Gyrase is a type II topoisomerase and the only enzyme that can catalyse the introduction of negative supercoils into DNA;3,5 it is composed of two subunits, GyrA and GyrB, which form an A2B2 complex in the active enzyme. Gyrase is an essential enzyme in bacteria and has been extensively studied as a target for antibacterial agents;6 gyrase has been described as an effective drug target for the development of new anti-TB agents. Other compounds, such as the aminocoumarins (e.g. novobiocin), inhibit gyrase through targeting the ATPase domains of gyrase and topo IV, located in the N-terminal domain of GyrB (and ParE), thus preventing supercoiling. In addition, we present crystal structures of the GyrB N-terminal ATPase sub-domain from Mycobacterium thermoresistibile bound to one of these compounds (Redx03863) and also to novobiocin, demonstrating that this novel compound class inhibits via a binding pocket and resistance mechanism different from that of novobiocin.

Using cross-seeding from crystals of the novobiocin complex, crystals of Redx03863 bound to the 21 kDa fragment were obtained, which diffracted to a resolution of 1.5 Å. The structure was solved using molecular replacement from the novobiocin complex structure. This new crystal structure demonstrated that the binding mode of Redx03863 partially overlaps those of novobiocin and 5′-adenylyl-β,γ-imidodiphosphate (ADPNP). However, in contrast to novobiocin, Redx03863, is more deeply buried and shows a greater correspondence in atomic positions to ADPNP, most notably in the overlap of the pyrrolopyrimidine and adenine rings. In the Redx03863 complex, there is only a water-mediated interaction between Arg141 and the ligand. Indeed, when we made site-directed mutations to Ala and Gln at Arg141 in M. tuberculosis GyrB, the mutated proteins showed only weak supercoiling activity and were susceptible to inhibition by Redx03863, i.e. this water-mediated contact does not greatly affect the interaction of Redx03863 with gyrase. When we selected for spontaneous resistance mutations to Redx03863 in M. smegmatis, the only mutation that we could isolate was Gly83Ser; no mutations at Arg141 were found, again suggesting it is of minor importance. In relation to Gly83 to Ser, the presence of a side chain at this position would cause steric clashes with the neighbouring structure and most likely displace and/or destabilize the loop bearing residue 83, which also contains several other important ligand-binding residues, namely Arg82, Ile84 and Pro85. We found that none of these mutant enzymes showed any supercoiling activity. This suggests that selecting resistance mutations to Redx03863 is difficult without compromising enzyme activity, which is a feature in favour of exploiting these compounds as leads for antimicrobial chemotherapy.

>[2x]GMLEGLEAVRKRPGMYIGSTGERGLHHLIWEVVDNAVDEAMAGHATKVRVRLLADGGVEVSDDGRGIPVEMHESGVPTVDVVMTQVGVSVVNALSTRMEVEICRDGYQWFQTYDKSVPGTLKQGEKTRKTGTVVRFWPDPDVFETTTFDFETVARRLQEQAFLNKGLTIELIDERDGKHRTFYYPG> RGRKRHCKTK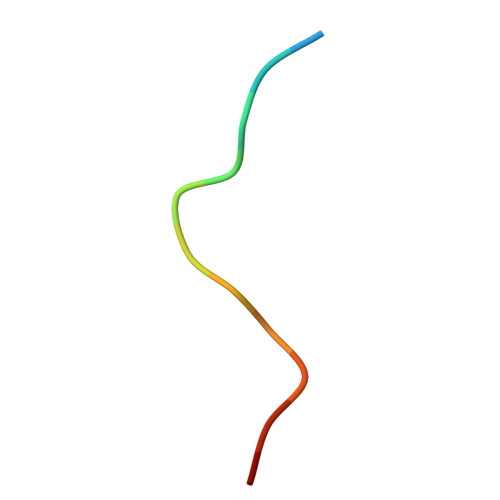HLE> GAMEGFKANLSLLRRPGEKTYTQRCRLFVGNLPADITEDEFKRLFAKYGEPGEVFINKGKGFGFIKLESRALAEIAKAELDDTPMRGRQLRVRFATHAAALSVRNLSPYVSNELLEEAFSQFGPIERAVVIVDDRGRSTGKGIVEFASKPAARKAFERCSEGVFLLTTTPRPVIVEPLEQLDDEEGLPEKLVIKNQQFHKEREQPPRFAQ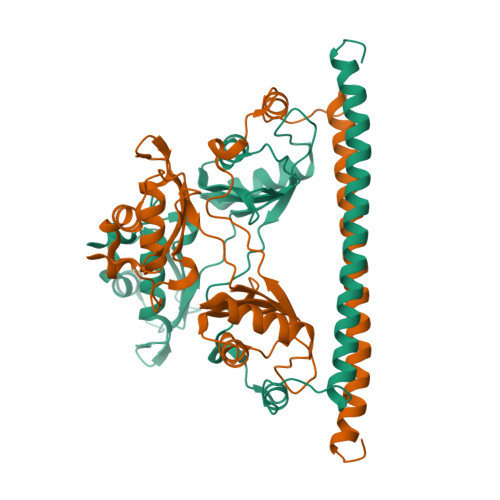PGSFEYEYAMRWKALIEMEKQQREQVEKNMKDAKDKLESEMEDAYHEHQANLL> MKILVIQGPNLNMLGHRDPRLYGMVTLDQIHEIMQTFVKQGNLDVELEFFQTNFEGEIIDKIQESVGSDYEGIIINPGAFSHTSIAIADAIMLAGKPVIEVHLTNIQAREEFRKNSYTGAACGGVIMGFGPLGYNMALMAMVNILA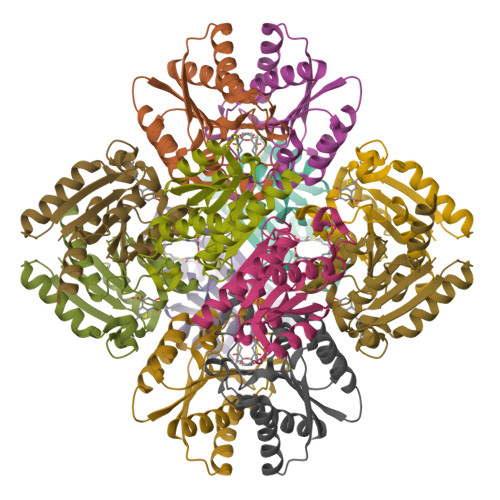EMKAFQEAQKNNPNNPINNQK>[4x]MSLKITDVDVWVVNLPLVNPFTSSFETKTGETRTVVRVRTDSGVEGWGETMWGAPVAAIVRRMAPDLIGTSPFALEAFHRKQHMVPFFYGYLGYAAIAAVDVACWDAMGKATGQSVTDLLGGAVRDEVPITALITRADAPGATPADLPKAMAEHAVRVVEEGGFDAVKLKGTTDCAGDVAILRAVREALPGVNLRVD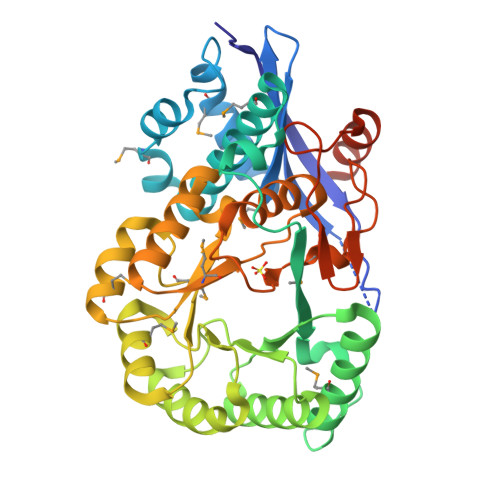PNAAWSVPDSVRAGIALEELDLEYLEDPCVGIEGMAQVKAKVRIPLCTNMCVVRFEDFAPAMRLNAVDVIHGDVYKWGGIAATKALAAHCETFGLGMNLHSGGELGIATAAHLAVVSSTPVLSRAIDSMYYLHADDIIEPLHLENGRLRVPSGPGLGVSVDEDKLRHYAGVNERDGDLTGEGHHHHHH Bgl1 catalyses the final step of in the decomposition of cellulose, an unbranched glucose polymer that has attracted the attention of researchers in recent years as it is the most abundant renewable source of reduced carbon in the biosphere. Bgl1 is a member of glycosyl hydrolase family 1 (GH1 superfamily, EC 3.2.1.21) and the results showed that the 3D structure of Bgl1 follows the overall architecture of the GH1 family, with a classical (β/α)8 TIM-barrel fold. Bgl1 has a half-life of 250 h at 60°C and it has been shown to be a thermostable enzyme with a broad substrate specificity and saccharification ability that efficiently hydrolyses cellooligosaccharides to glucose. The catalytic site residues of the enzyme are two glutamic acid residues, Glu163 and Glu361, as in other enzymes that belong to the same family.

Here, we report the three-dimensional structures of Bgl1 from the thermophilic bacterium C. saccharolyticus and its complex with glucose, which is the product of its catalytic action when lactose is used as a substrate, that were determined at 1.47 and 1.95 Å resolution, respectively. The Bgl1 crystals grew in the monoclinic space group P21with two molecules per asymmetric unit. Comparison of the two monomers in each individual structure showed that they have negligible differences, with an r.m.s.d. on Cα atoms or secondary-structure elements of 0.16 Å for Bgl1. In the case of Bgl1, sufficient electron density to accommodate a glycerol (GOL) molecule and an ethylene glycol (EDO) molecule was observed at the active site of the enzyme and both were added to the model, which was then subjected to refinement. Both molecules form hydrogen bonds and van der Waals interactions with the catalytic residues Glu361 and Glu163, respectively, and mimic the binding mode of the substrate. An additional glycerol molecule is bound at the interface of the first monomer (chain A) with a symmetry-related molecule of the second monomer (chain B; symmetry operator −x, y + 1/2, −z). The 2Fobs − Fcalc and Fobs − Fcalc electron-density maps also revealed the binding of polyethylene glycol (PEG) molecules that lie on the surface of the Bgl1 structure in those areas which are most exposed to the solvent and are not involved in symmetry-related packing interactions.

>[2x]SHMLEDPMSFPKGFLWGAATASYQIEGAWNEDGKGESIWDRFTHQKRNILYGHNGDVACDHYHRFEEDVSLMKELGLKAYRFSIAWTRIFPDGFGTVNQKGLEFYDRLINKLVENGIEPVVTLYHWDLPQKLQDIGGWANPEIVNYYFDYAMLVINRYKDKVKKWITFNEPYCIAFLGYFHGIHAPGIKDFKVAMDVVHSLMLSHFKVVKAVKENNIDVEVGITLNLTPVYLQTERLGYKVSEIEREMVSLSSQLDNQLFLDPVLKGSYPQKLLDYLVQKDLLDSQKALSMQQEVKENFIFPDFLGINYYTRAVRLYDENSSWIFPIRWEHPAGEYTEMGWEVFPQGLFDLLIWIKESYPQIPIYITENGAAYNDIVTEDGKVHDSKRIEYLKQHFEAARKAIENGVDLRGYFVWSLMDNFEWAMGYTKRFGIIYVDYETQKRIKKDSFYFYQQYIKENS>GSKEGEYIKLKVIGQDSSEIHFKVKMTTHLKKLKESYAQRQGVPMNSLRFLFEGQRIADNHTPKELGMEEEDVIEVYQEQTGG[2x];>G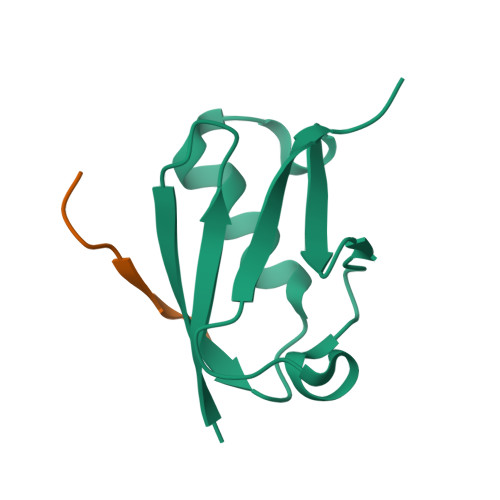SGEAEERIISLD[2x]> KDVPPKQLRFEGERVTWIQASTLKELLDLKAQHPEAKLVVGNTEIGIEMKFKNQLFPMIICPAWIPELNAVEHGPEGISFGAACALSSVEKTLLEAVAKLPTQKTEVFRGVLEQLRWFAGKQVKSVASLGGNIITASPISDLNPVFMASGTKLTIVSRGTRRTVPMDHTFFPSYRKTLLGPEEI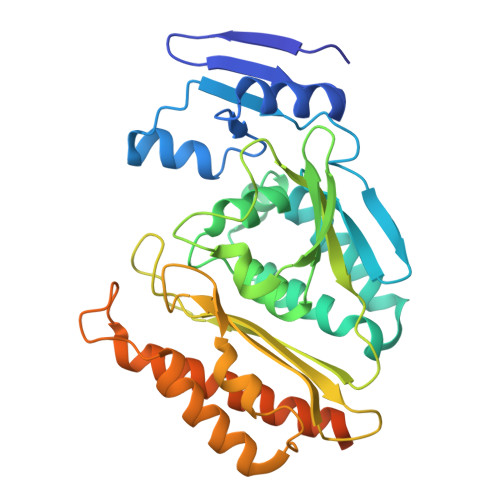LLSIEIPYSREDEFFSAFKQASRREDDIAKVTCGMRVLFQPGSMQVKELALCYGGMADRTISALKTTQKQLSKFWNEKLLQDVCAGLAEELSLSPDAPGGMIEFRRTLTLSFFFKFYLTVLKKLGKDSKDKCGKLDPTYTSATLLFQKDPPANIQLFQEVPNGQSK TRPV5 is a calcium selective ion channel that is responsible for the fine tuning of calcium reabsorption in the kidney and has been shown to be a critical component of systemic calcium homeostasis. In the cell, binding of PI(4,5)P2 is critical for channel opening while rapid desensitization occurs via binding of calmodulin (CaM) to the base of the pore. The transmembrane domain (TMD) consists of transmembrane helices 1–4 (S1-S4) bundled in a voltage sensing-like domain with helices 5 and 6 (S5 and S6) domain swapped to create the pore of the channel. The intracellular portion of the protein is primarily composed of tightly packed ankyrin repeat domains (ARDs).

The fifth derivative, ZINC17988990, was found to be a potent inhibitor of TRPV5 mediated currents. This compound exhibited robust inhibition of rbTRPV5 with an IC50 of 106 ± 27 nM while also showing marked selectivity for TRPV5 over TRPV6. In order to verify that the newly identified TRPV5 inhibitors, ZINC9155420 and ZINC17988990, bind to TRPV5, we utilized cryo-electron microscopy (cryo-EM) to solve the structure of rabbit TRPV5 in the presence of each compound. We were able to resolve nanodisc-reconstituted TRPV5 in the presence of 10 µM ZINC9155420 or ZINC17988990 to 4.3 Å and 3.8 Å, respectively (Figure 3—figure supplements 1–4). At these resolutions, we were able to clearly identify that the ion conduction pathway for both inhibitor-bound structures are in non-conducting conformations. The ZINC17988990-bound TRPV5 structure revealed two densities that could be attributed to bound compounds. One density identified in the ZINC17988990-bound TRPV5 structure is located between the intracellular S1-S4 bundle and the TRP helix and it is present in the sharpened map as well as both of the half-maps. Though the upper region of the S1-S4 pocket has been consistently occupied by lipids in the previous TRPV5 channel structures, a density lower in the pocket has been identified for the first time in the ZINC17988990-bound structure. In the case of TRPV6, this was proposed in spite of lipid binding reported in the same area in previous structures. This precedent, along with the absence of the lower density in previously published TRPV5 cryo-EM structures, has led us to attribute this density to bound ZINC17988990. The residues that constitute this binding site in the S1-S4 bundle of the ZINC17988990-bound TRPV5 structure include E403, D406, Y415, Y467 and F468. The substantially reduced inhibitory effects of these S1-S4 bundle mutant channels indicate that this compound exerts its inhibitory effect primarily by binding in this pocket. Specifically, the S2 and S3 helices of the ZINC17988990-bound TRPV5 have moved toward the ZINC17988990 density, which creates a tighter space with in the intracellular section of the S1-S4 bundle compared to the lipid-bound apo TRPV5 structure.

>[4x]MGACPPKAKGPWAQLQKLLISWPVGEQDWEQYRDRVNMLQQERIRDSPLLQAAKENDLRLLKILLLNQSCDFQQRGAVGETALHVAALYDNLEAATLLMEAAPELAKEPALCEPFVGQTALHIAVMNQNLNLVRALLARGASVSARATGAAFRRSPHNLIYYGEHPLSFAACVGSEEIVRLLIEHGADIRAQDSLGNTVLHILILQPNKTFACQMYNLLLSYDEHSDHLQSLELVPNHQGLTPFKLAGVEGNTVMFQHLMQKRKHVQWTCGPLTSTLYDLTEIDSWGEELSFLELVVSSKKREARQILEQTPVKELVSFKWKKYGRPYFCVLASLYILYMICFTTCCIYRPLKLRDDNRTDPRDITILQQKLLQEAYVTHQDNIRLVGELVTVTGAVIILLLEIPDIFRVGASRYFGQTILGGPFHVIIITYASLVLLTMVMRLTNMNGEVVPLSFALVLGWCSVMYFARGFQMLGPFTIMIQKMIFGDLMRFCWLMAVVILGFASAFHITFQTEDPNNLGEFSDYPTALFSTFELFLTIIDGPANYSVDLPFMYCITYAAFAIIATLLMLNLFIAMMGDTHWRVAQERDELWRAQVVATTVMLERKMPRFLWPRSGICGYEYGLGDRWFLRVENHHDQNPLRVLRYVEAFKCSDKEDGQEQLSEKRPSTVESGMLSRASVAFQTPSLSRTTSQSSNSHRGWEILRRNTLGHLNLGLDLGEGDGEEVYHF>GGGACCAGGGGUGCUUGUUCACAGGCUGAGAAAGUCCCUUUGAACCUGAACAGGGUAAUGCCUGCGCAGGGAGU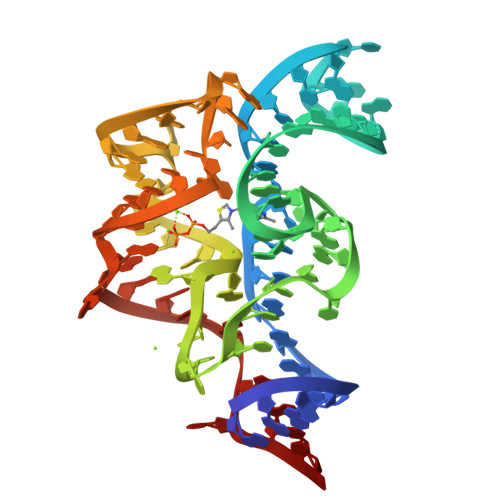GUC[2x]> TTVNETTPIAPAKVLPDAQTVTSVRHWTDTLFSFRVTRPQTLRFRSGEFVMIGLLDDNGKPIMRAYSIASPAWD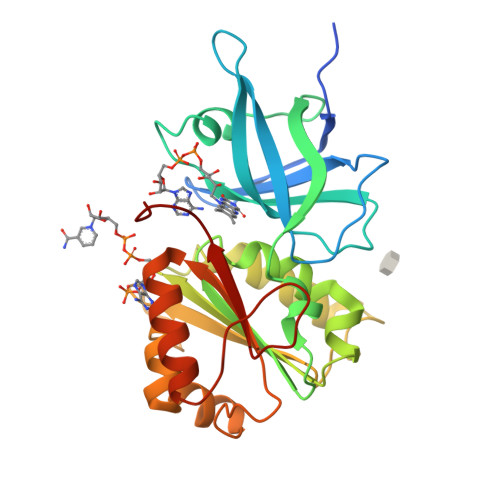EELEFYSIKVPDGPLTSRLQHIKVGEQIILRPKPVGTLVIDALLPGKRLWFLATGTGIAPFASLMREPEAYEKFDEVIMMHACRTVAELEYGRQLVEALQEDPLIGELVEGKLKYYPTTTREEFHHMGRITDNLASGKVFEDLGIAPMNPETDRAMVCGSLAFNVDVMKVLESYGLREGANSEPREFVVEKAFVGEGI> MSDSKEVPSLPFLRHLLEELDSHEDSLLLFLCHDAAPGCTTVTQALCSLSQQRKLTLAALVEMLYVLQRMDLLKSRFGLSKEGAEQLLGTSFLTRYRKLMV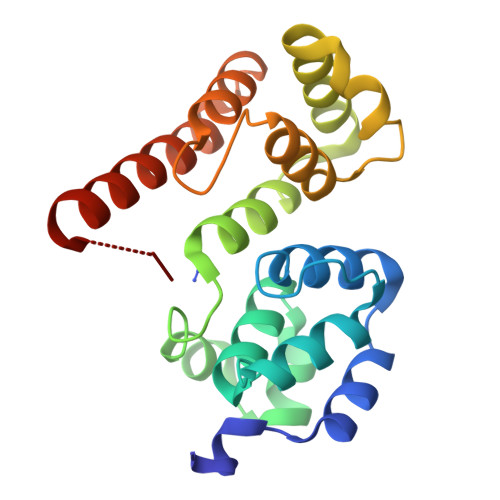CVGEELDSSELRALRLFACNLNPSLSTALSESSRFVELVLALENVGLVSPSSVSVLADMLRTLRRLDLCQQLVEYEQQEQARYRYCLEHHHHHH>GPLGSPEFQKTKPFSVPNLPLNTLSNSRVPSLIRSMMVSRDHGQMVQFQNGRVTLDGQLQGTTPTSASQLCKIRGSVFHANGGNGYNLTELDGSPYHAFESPAPIGFPDLGECDWHMEASPTTQFDTGDVIKQINVKQEAAFAPHLGTIQADGLSDVSVNTNMIAKLGWVSPASDGHRGNVDPWVIPRYGSTLTEAAQLAPPIYPPGFGEAIVFFMSDFPIAHGANGLSVPCTIPQEFVTHFVNEQAPTRGEAALLHYLDPDTHRNLGEFKLYPEGFMTCVPNSSGTGPQTLPINGVFVFVSWVSRFYQLKPVGTAGPARSLGIRRS[4x]

NoV VP1 can be divided into two major domains: the N-terminal shell (S) domain and the C-terminal protruding (P) domain. The P domains form the outermost, dimeric protrusions of NoV virions, which plays critical roles in receptor recognition and host immune responses. HuNoVs recognize human histo-blood group antigens (HBGAs) as host receptors or attachment factors that play an important role in huNoV host susceptibility. In this study, we provided both phenotypic and structural evidence to show that huNoV DSV and VA115 recognize a group of glycans with terminal galactoses as ligands.

The results showed that two oligosaccharides (117 and 373) bound well to both DSV/VA115 P-GST fusion proteins with significantly higher binding signals compared with the remaining 583 oligosaccharides. Interestingly, only one oligosaccharide molecule bound in each asymmetric unit of the complex structures, since the remaining oligosaccharide binding pockets contain steric hindrance for oligosaccharides at crystal packing interface. The positions of the glycan binding pockets were located at the outermost surface of the P protein near the interface between the two P monomers, similar to the typical HBGA binding sites of other GI huNoVs. The binding interface of VA115 P protein resembles that of DSV, in which its “bottom” is also composed of the four conserved residues D332, H334, S389, and P390. Similarly, in VA115 the Gal forms five direct hydrogen bonds with four conserved amino acids, D332, H334, S389, and P390, as well as G394 at the position corresponding to Q393 of the DSV P protein that does not participate in direct interaction. P390A of VA115 was the only mutation that did not change the glycan binding ability of the mutant P protein, presumably because this residue interacts with the trisaccharide through its main chain carbonyl group. The structural data showed that the two GI.3 huNoVs bound non-HBGA glycans using terminal Gal as the MaBS, explaining the mechanism why these huNoVs could not bind HBGAs.>[2x]SSSHPIFHRGEFSVCDSVSVWVGDKTTATDIKGKEVMVLGEVNINNSVFKQYFFETKCRDPNPVDSGCRGIDSKHWNSYC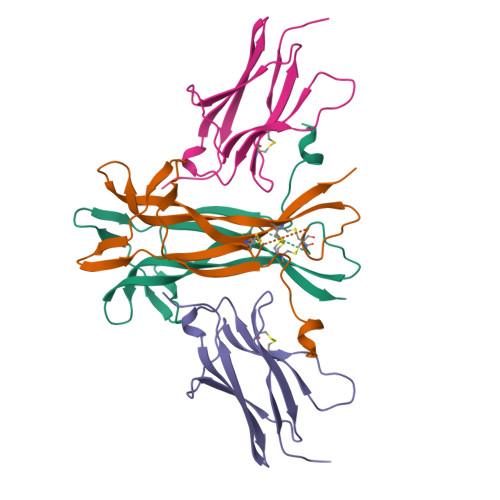TTTHTFVKALTMDGKQAAWRFIRIDTACVCVLSRKAVRRA;>VSFPASVQLHTAVEMHHWCIPFSVDGQPAPSLRWLFNGSVLNETSFIFTEFLEPAANETVRHGCLRLNQPTHVNNGNYTLLAANPFGQASASIMAAFMDNP[2x]>MGPGFDFAQAIMKKNTVIARTEKGEFTMLGVYDRVAVIPTHASVGEIIY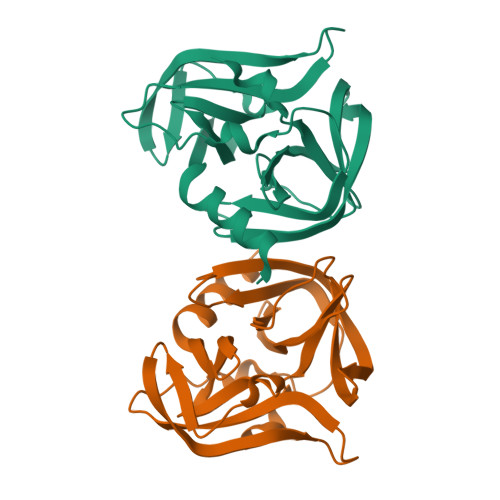INDVETRVLDACALRDLTDTNLEITIVKLDRNQKFRDIRHFLPRCEDDYNDAVLSVHTSKFPNMYIPVGQVTNYGFLNLGGTPTHRILMYNFPTRAGQCGGVVTTTGKVIGIHVGGNGAQGFAAMLLHSYFTDTQKHHHHHH[2x]(2R)-2-amino-N-{(2S)-1-[(4-carbamimidoylbenzyl)amino]-1-oxopropan-2-yl}-4-(4-hydroxyphenyl)butanamide 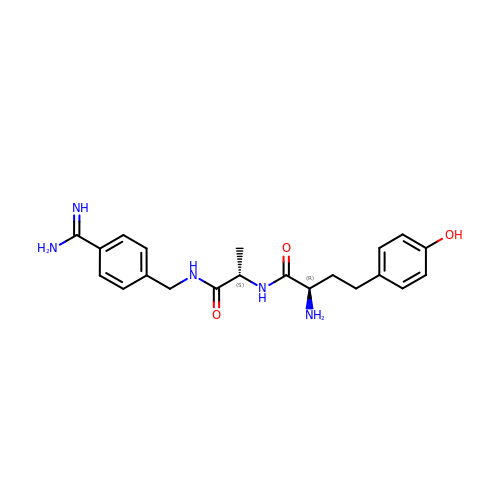| C21 H27 N5 O3 | GVEMEQSTGJKMAX-SCLBCKFNSA-N Here, using functional metagenomic selection, we describe AcrIIA22, an unconventional Acr found in hypervariable genomic regions of clostridial bacteria and their prophages from human gut microbiomes. AcrIIA22 encodes a 54 amino acid protein that impairs SpyCas9 activity. Instead, guided by an X-ray crystal structure of AcrIIA22, coupled with mutational and biochemical analyses, we show that AcrIIA22 encodes a DNA nickase. By nicking a supercoiled plasmid substrate and relieving its torsional stress, AcrIIA22 renders the target less susceptible to SpyCas9 activity.

Anticipating that structural homology might provide better insight into its mechanism of inhibition, we solved AcrIIA22’s structure using X-ray crystallography. The asymmetric unit in AcrIIA22’s crystal comprises 2 monomers stacked end to end, with each monomer folding into a 4-stranded β-sheet. A DALI structure–structure search revealed that the AcrIIA22 monomer is similar to members of the newly recognized PC4-like structural fold. Despite crystallizing as a homodimer, AcrIIA22 migrated from a size exclusion chromatography (SEC) column at an elution volume corresponding to a calculated mass approximately 4 times larger than its expected monomeric molecular weight. Indeed, AcrIIA22 was predicted to form a stable tetramer when analyzed with PISA, a tool for inferring macromolecular assembles from crystal structures. This putative tetramer has a molecular mass consistent with that observed by SEC and comprises pairs of outward-facing, concave β-sheets. A series of hydrophobic interactions likely stabilize this configuration of β-sheets instead of the typical α-helical interactions seen in other PC4-like proteins, potentially explaining the absence of an α-helix in AcrIIA22. Consistent with this possibility, AcrIIA22’s β-sheets orient along each outward face of the putative tetramer, resemble those in PC4-like proteins, and form a groove that could potentially accommodate a nucleic acid substrate. Our tetramer model predicts that an interface at the C-terminus of AcrIIA22 is required for adjacent β-sheets to bind one another and form a grooved, oligomeric structure. Instead, we speculate that D14 may contribute to AcrIIA22’s nicking activity, as 2 D14 residues from different AcrIIA22 monomers sit very near to one another in our proposed tetramer, such that they may be stabilized via the presence of a divalent cation under physiological conditions.

>[2x]GSSMGMVVEETRDLAETADCVVIEAILVDDGLRYRQLSVGIKDENGDIIRIVPISTVLI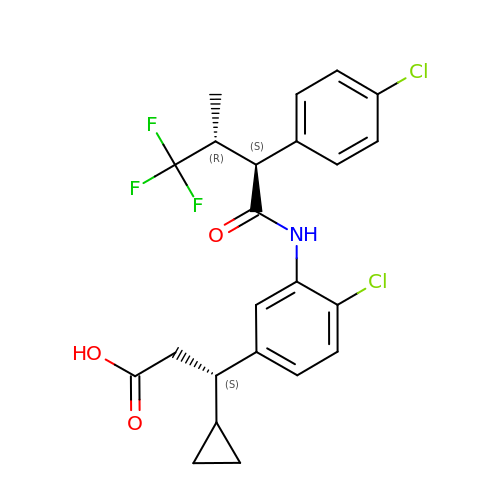Runcaciguat | C23 H22 Cl2 F3 N O3 | NCRMKIWHFXSBGZ-CNBXIYLPSA-N>[3x]GAMGMNTPPELDTVLQAPYAYNWPTSKNVKIASRIGIPY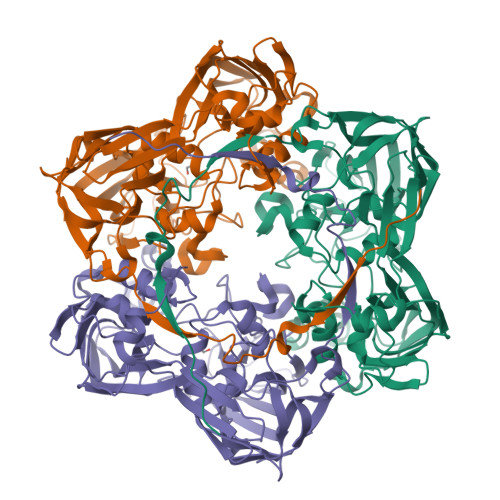STFQTIQPVSDAPNNGIGQITFNQPLGNLTGGAPRLRVSFTAEIKNILADSSLKDQIGLKSFPVNRSIPVAVINMNGKTFTSYPAQLIKLHQYNADPLELALLSPCSDVDEYNKIKAVSMNNPYRQGTESTDSRMSRGLGCNYAYYIHPRAAGSTSVKIDFVVDEALVANPTQYKNIKDPVPFRNLNTFKVILDGQFKPENMIGIADDVKLVAGKADFEVDITGFKINMLVQNWVAPLEIGDIPKTIIYNTPLISLEGNISSMCLNTKDPYGIPGERNKHILTTHSMAMNNVPSMFAVMVSQETPTKKFAPDQLAGIIGLEIKVDSDVGIFRELEQQQLYELSSSNGYNKRFSCFSGALANGLTVADPAVAAGNKFKEAIFGAGSVIFFRPSDLGLKDYNVMANANKSINMQVQATFVTPEAAGTGAHYKLEVFSIRDNLTYSFEDGTFMDDLTLYTPDQLLRSPLKLTDDNNKLMRVMGGSFMGDVMTNFNHMAAHPVTKTVTKLLRNAGPLKDYAGDGTMMGNIASVYGYGKKKTTTRKKKGGEIVLLGSGKKGGKKLSDKQLHDLRNL> MDLSGKMV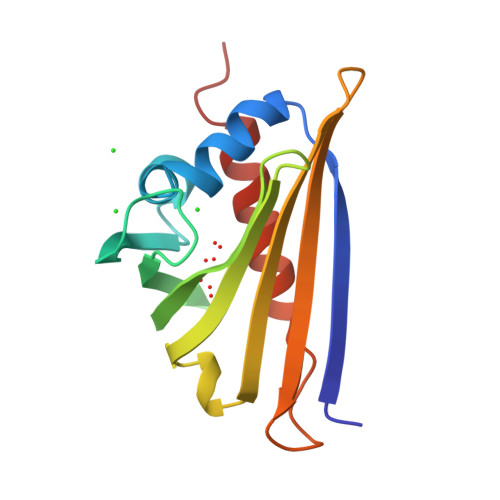KQVEILSDGIVFYEIFRYRLYLISEMSPVNIQGVDLLEGNWGTVGSVIFFKYTIDGKEKTAKDIVEAIDEETKSVTFKIVEGDLMELYKTFIIIVQVDTKGEHNSVTWTFHYEKLKEDVEEPNTLMNFCIEITKDIETYHLK>[4x]ETGTPMMPPVGVQASILSHDTIRITWADNSLPKHQKITDSRYYTVRWKTNIPANTKYKNANATTLSYLVTGLKPNTLYEFSVMVTKGRRSSTWSMTAHG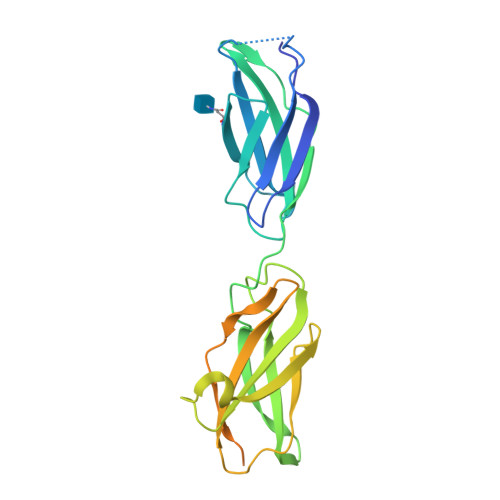ATFELVPTSPPKDVTVVSKEGKPRTIIVNWQPPSEANGKITGYIIYYSTDVNAEIHDWVIEPVVGNRLTHQIQELTLDTPYYFKIQARNSKGMGPMSEAVQFRTPKADSSDKMPNDQALGSAGKGSRLPDLGSDYKPPMSGSNSPHGSPTSPLDSNGTKHHHHHH> MGHHHHHHHHHHSSGHIDDDDKHM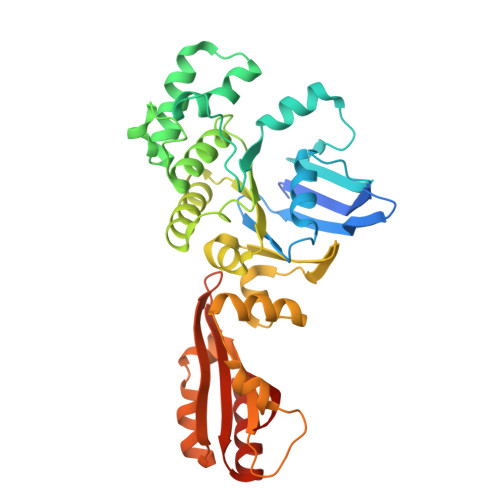IKLSNITKVFHQGTRTIQALNNVSLHVPAGQIYGVIGASGAGKSTLIRCVNLLERPTEGSVLVDGQELTTLSESELTKARRQIGMIFQHFNLLSSRTVFGNVALPLELDNTPKDEVKRRVTELLSLVGLGDKHDSYPSNLSGGQKQRVAIARALASNPKVLLCDQATSALDPATTRSILELLKDINRRLGLTILLITHEMDVVKRICDCVAVISNGELIEQDTVSEVFSHPKTPLAQKFIQSTLHLDIPEDYQERLQAEPFTDCVPMLRLEFTGQSVDAPLLSETARRFNVNNNIISAQMDYAGGVKFGIMLTEMHGTQQDTQAAIAWLQEHHVKVEVLGYV> MRHPFKVVVVTGVPGVGKTTVIKELQGLAEKEGVKLHIVNFGSFMLDTAVKLGLVEDRDKIRTLPLRRQLELQREAAKRIVAEASKALGGDGVLIIDTHALVKTVAGYWPGLPKHVLDELKPDMIAVV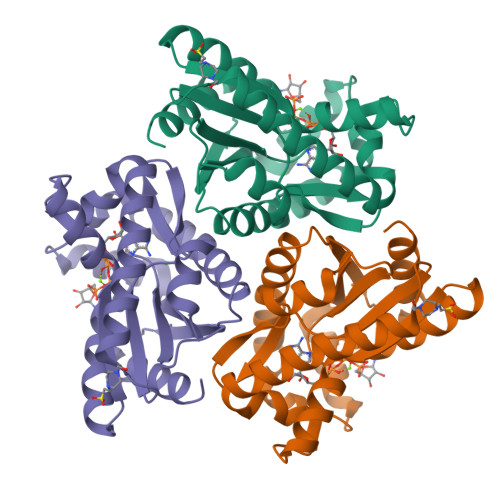EASPEEVAARQARDTTRYRVDIGGVEGVKRLMENARAASIASAIQYASTVAIVENREGEAAKAAEELLRLIKNL>ASASVLDYLELADEHSIVELKATEKMAGQSIIDLDIRAQYGINIIAIKRGKEFIISPNPNINLEIGDILIMIGHDNDLNRFEKN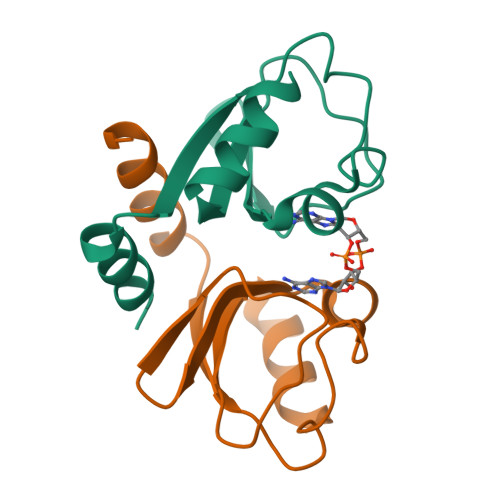I[2x]>MIKVNELLDKINRKRSGDTLLLTNISFMSFSEFRHRTSGTLTWRETDFLYQQAHQESKQNKLEELRILSRANPQLANITNLNITPSTLNNSYNSWFYGRAHRFVKPGSIASIFSPAAYLTELYREAKDFHPDNSQYHLNKRRPDIASLALTQNNMDEEISTLSLSNELLLHNIQTLEKTDYNGVMKMLSTYRQTGMTPYHLPYESARQAILLQDKNLTAFSRNTDVAELMDPTSLLAIKTDISPELYQILVEEITPENSTELMKKNFGTDDVLIFKSYASLARYYDLSYDELSLFVNLSFGKKNTNQQYKNEQLITLVNDGNDTATARLIKRTRKDFYDSHLNYAELIPIKENEYKYNFSVKKTEPDHLDFRLQNGDKEYIYQDKNFVPIANTHYSIPIKLTTEQITNGITLRLWRVKPNPSDAINANAHFKMMEFPGDIFLLKLNKAIRLYKATGISPEDIWQVIESIYDDLTIDSNVLGKLFYVQYYMQHYNISVSDALVLCHSDISQYSTKQQPSHFTMLFNTPLLNGQEFSADNTKLDLTPGESKNHFYLGIMKRAFRVNDTELYTLWKLANGGTNPEFMCSIENLSLLYRVRLLADIHHLTVNELSMLLSVSPYVNTKIALFSDTALTQLISFLFQCTQWLTTQKWSVSDVFLMTTDNYSTVLTPDIENLITTLSNGLSTLSLGDDELIRAAAPLIAASIQMDSAKTAETILLWINQIKPQGLTFDDFMIIAANRDRSENETSNMVAFCQVLGQLSLIVRNIGLSENELTLLVTKPEKFQSETTALQHDLPTLQALTRFHAVIMRCGSYATEILTALELGALTAEQLAVALKFDAQVVTQALQQTDLGVNTFTNWRTIDVTLQWLDVAATLGITPDGVAALIKLKYVGEPETPMPTFDDWQAASTLLQAGLNSQQSDQLQAWLDEATTTAASAYYIKNGAPQQIKSRDELYSYLLIDNQVSAQVKTTRVAEAIASIQLYVNRALNNVEGKVSKPVKTRQFFCDWETYNRRYSTWAGVSELAYYPENYIDPTIRIGQTGMMNNLLQQLSQSQLNIDTVEDSFKNYLTAFEDVANLQVISGYHDSINVNEGLTYLIGYSQTEPRIYYWRNVDHQKCQHGQFAANAWGEWKKIEIPINVWQENIRPVIYKSRLYLLWLEQKELKNESEDGKIDITDYILKLSHIRYDGSWSSPFNFNVTDKIENLINKKASIGMYCSSDYEKDVIIVYFHEKKDNYSFNSLPAREGMTINPDMTLSILTENDLDAIVKSTLSELDTRTEYKVNNQFATDYLAEYKESITTKNKLASFTGNIFDLSYISPGNGHINLTFNPSMEINFSKGNIYNDEVKYLLSMVEDETVILFDYDRHDEMLGKEEEVFHYGTLDFIISIDLKNAEYFRVLMHLRTKEKIPRKSEIGVGINYDYESNDAEFKLDTNIVLDWKDNTGVWHTICESFTNDVSIINNMGNIAALFLREDPCVYLCSIA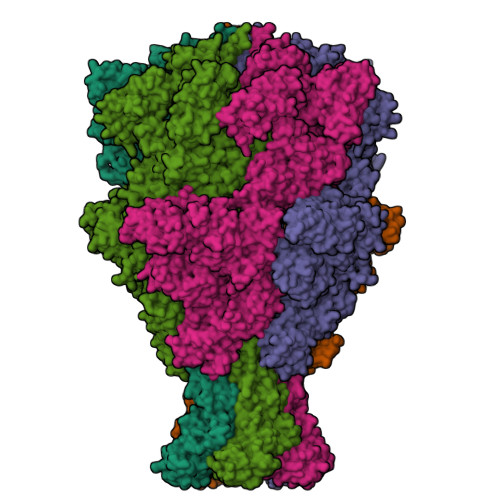TDIKIASSMIEQIQDKNISFLLKNGSDILVELNAEDHVASKPSHESDPMVYDFNQVKVDIEGYDIPLVSEFIIKQPDGGYNDIVIESPIHIKLKSKDTSNVISLHKMPSGTQYMQIGPYRTRLNTLFSRKLAERANIGIDNVLSMETQNLPEPQLGEGFYATFKLPPYNKEEHGDERWFKIHIGNIDGNSARQPYYEGMLSDIETTVTLFVPYAKGYYIREGVRLGVGYKKIIYDKSWESAFFYFDETKNQFIFINDADHDSGMTQQGIVKNIKKYKGFIHVVVMKNNTEPMDFNGANAIYFWELFYYTPMMVFQRLLQEQNFTESTRWLRYIWNPAGYSVQGEMQDYYWNVRPLEEDTSWNANPLDSVDPDAVAQHDPMHYKVATFMKMLDLLITRGDSAYRQLERDTLNEAKMWYVQALTLLGDEPYFSLDNDWSEPRLEEAASQTMRHHYQHKMLQLRQRAALPTKRTANSLTALFLPQINKKLQGYWQTLTQRLYNLRHNLTIDGQPLSLSLYATPADPSMLLSAAITASQGGGDLPHAVMPMYRFPVILENAKWGVSQLIQFGNTLLSITERQDAEALAEILQTQGSELALQSIKMQDKVMAEIDADKLALQESRHGAQSRFDSFNTLYDEDVNAGEKQAMDLYLSSSVLSTSGTALHMAAAAADLVPNIYGFAVGGSRFGALFNASAIGIEISASATRIAADKISQSEIYRRRRQEWEIQRNNAEAEIKQIDAQLATLAVRREAAVLQKNYLETQQAQTQAQLAFLQSKFSNAALYNWLRGRLSAIYYQFYDLAVSLCLMAEQTYQYELNNAAAHFIKPGAWHGTYAGLLAGETLMLNLAQMEKSYLEKDERALEVTRTVSLAEVYAGLTENSFILKDKVTELVNAGEGSAGTTLNGLNVEGTQLQASLKLSDLNIATDYPDGLGNTRRIKQISVTLPALLGPYQDVRAILSYGGSTMMPRGCKAIAISHGMNDSGQFQMDFNDAKYLPFEGLPVADTGTLTLSFPGISGKQKSLLLSLSDIILHIRYTIRS[5x]>[2x]MDYLVKALAYDGKVRAYAARTTDMVNEGQRRHGTWPTASAALGRTMTASLMLGAMLKGDDKLTVKIEGGGPIGAIVADANAKGEVRAYVSNPQVHFDLNAAGKLDVRRAVGTNGTLSVVKDLGLREFFTGQVEIVSGELGDDFTYYLVSSEQVPSSVGVGV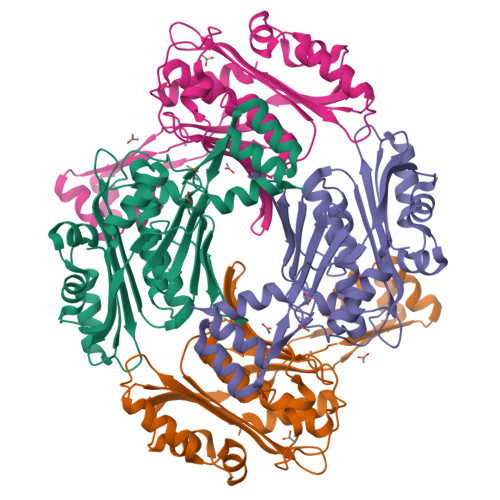LVNPDNTILAAGGFIIQLMPGTDDETITKIEQRLSQVEPISKLIQKGLTPEEILEEVLGEKPEILETMPVRFHCPCSKERFETAILGLGKKEIQDMIEEDGQAEAVCHFCNEKYLFTKEELEGLRDQTTR>[4x]XLAACLA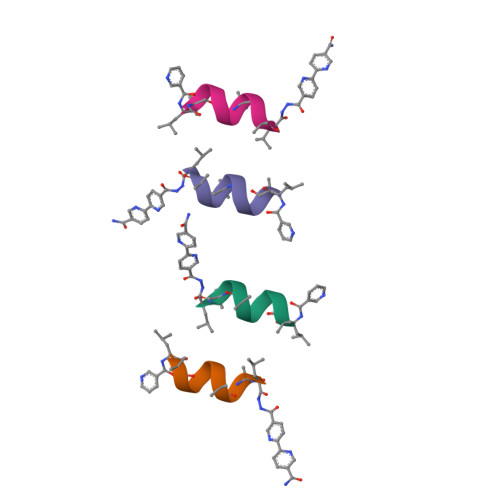CALX>GSPHMTKAEKILARFNELPNYDLKAVCTGCFHDGFNEVDIEILNQLGIKIFDNIKETDKLNCIFAPKILRTEKFLKSLSFEPLKFALKPEFIIDLLKQIHSKKDKLSQININLFDYEINGINESIISKTKLPTKVFERANIRCINLV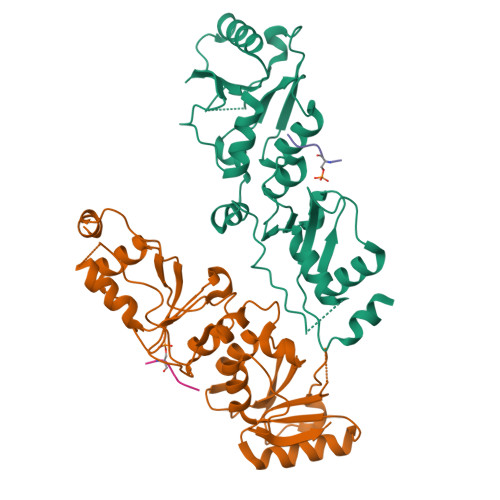NDIPGGVDTIGSVLKAHGIEKINVLRSKKCTFEDIIPNDVSKQENGGIFKYVLIVTKASQVKKFTKLINDRDKNETILIVEWNWCVESIFHLNVDFTSKKNVLYQKKNN[2x];>ATKASQEL[2x]N-methyl-1-[5-(pyridin-3-yloxy)furan-2-yl]methanamine | C11 H12 N2 O2 | 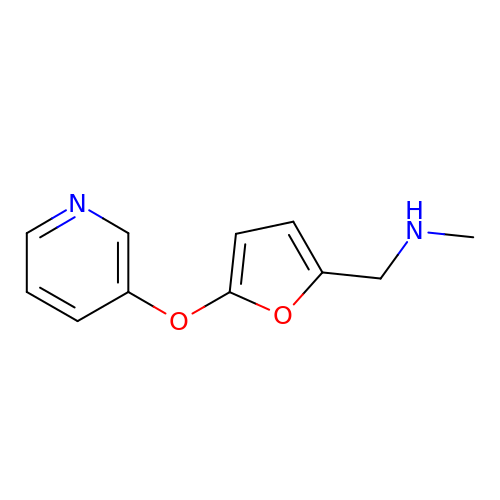MUKCVLFJCGZPKF-UHFFFAOYSA-N> CGAGGAAC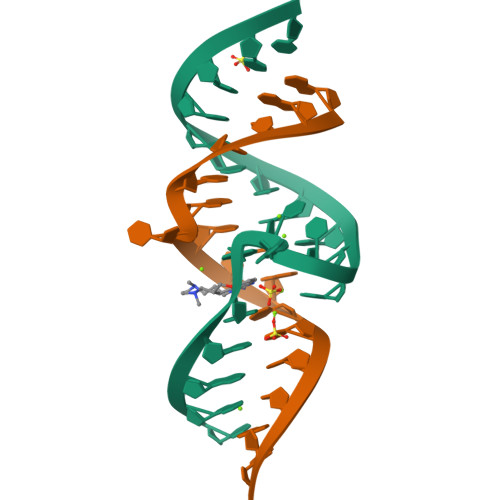UACUGUCUUCCC;> GGUCGUGCAGCCUCGG> TGMSREEVESLIQEVLEVYPEKARKDRNKHLAVNDPAVTQSKKCIISNKKSQPGLMTIRG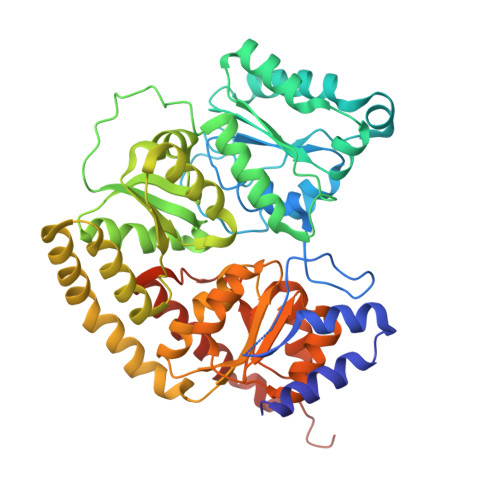CAYAGSKGIVWGPIKDMIHISHGPVGCGQYSRAGRRNYYIGTTGVNAFVTMNFTSDFQEKDIVFGGDKKLAKLIDEVETLFPLNKGISVQSECPIGLIGDDIESVSKVKGAELSKTIVPVRCEGFRGVSQSLGHHIANDAVRDWVLGKRDEDTTFASTPYDVAIIGDYNIGGDAWSSRILLEEMGLRCVAQWSGDGSISEIELTPKVKLNLVHCYRSMNYISRHMEEKYGIPWMEYNFFGPTKTIESLRAIAAKFDESIQKKCEEVIAKYKPEWEAVVAKYRPRLEGKRVMLYIGGLRPRHVIGAYEDLGMEVVGTGYEFAHNDDYDRTMKEMGDSTLLYDDVTGYEFEEFVKRIKPDLIGSGIKEKFIFQKMGIPFREMHSWDYSGPYHGFDGFAIFARDMDMTLNNPCWKKLQAPWEASEGAEKVAASA> NAVESTLRRVAKDLTGLRQRWALVGGFAVSARSEPRFTRDVDIVVAVANDDAAESLVRQLLTQQYHL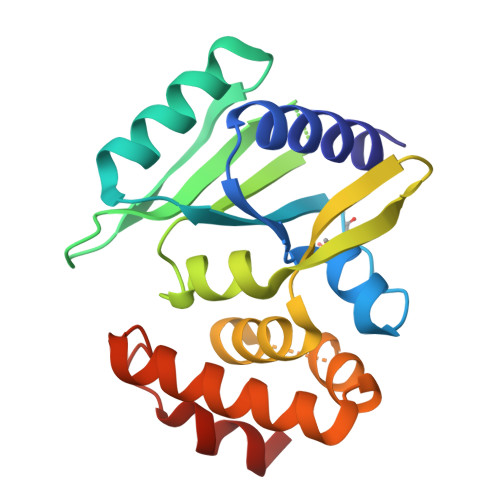LASVEQDAARRLAAVRLGATADTAANVVVDLLFASCGIEPEIAEAAEEIEILPDLVAPVATTAHLIAMKLLARDDDRRPQDRSDLRALVDAASPQDIQDARKAIELITLRGFHRDRDLAAEWTRLAAKW>[8x]ISHMIQNRAQAVDQLRAVARYFRQTEPHSPVAYLADKAAE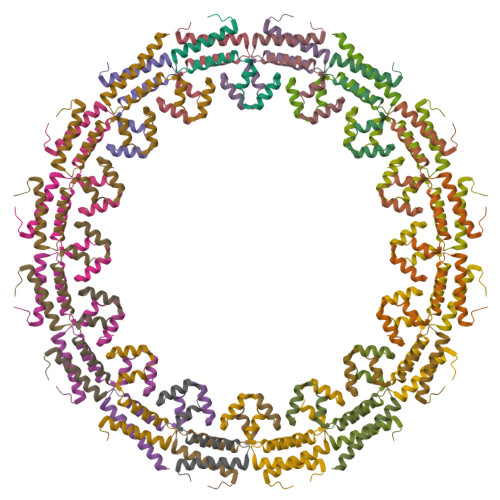WADMPLHKWLESVVKDDGSLSHIRELLGVRPDEQS>[3x]PMFIVNTNVPRASVPDGFLSELTQQLAQATGKPPQYIAVHVVPDQFMAFGGSSEPCALCSLHSIGKIGGAQNRSYSKLLCGLLAERLRISPDRVYINYYDMNAANVGWNNSTFA

Macrophage Migration Inhibitory Factor (MIF) is a ubiquitous multifunctional protein and a key player in the inflammatory response and innate immunity. MIF has two enzymatic activities: an evolutionarily well conserved keto-enol tautomerase activity and a thiol-protein oxido-reductase activity that is mediated by the C56ALC59 motif. X-ray structural studies have consistently shown that MIF exists as a homotrimer. Each MIF monomer consists of 114 amino acids and is composed of two anti-parallel α-helices packed against a four-stranded β-sheet.

To elucidate the role of intersubunit interactions involving Leu46 on the structure and stability of MIF, we compared the structural stability, and biophysical properties of wt, L46A, L46F and L46G mutants at the secondary, tertiary and quaternary structure levels. To understand the role of Leu46 mutations on the three-dimensional structure of MIF, we also determined the crystal structures of L46F, L46A and L46G huMIF at 1.70 Å, 1.70 Å and 1.60 Å, respectively. Similar to the wild type species, Leu46 mutants crystallized as homotrimeric proteins with dimensions of approximately 35 Å×50 Å×50 Å. In agreement with our previous structural studies, X-ray crystal structures of MIF variants demonstrate that the Leu46 mutants conserve the same three-dimensional structure pattern as the wt protein. Static light scattering, in agreement with the analytical ultracentrifugation data, demonstrated that wt, L46F, L46A and L46G exist as stable trimers. Finally, crystallographic data and enzymatic assays do not show any drastic conformational change of the catalytic site or activity of MIF upon Leu46 mutations. Using hydroxyphenylpyruvate as a substrate, we showed that all Leu46 mutants are enzymatically active. In our case, chemical shift measurements demonstrate an extremely high similarity between L46A and L46G huMIF, whereas the L46F mutant exhibits a slightly different chemical shift pattern. Taken together, our data suggest that the intersubunit interactions involving the residue Leu46 play a key role in the structural stability of MIF and provide new insights into the role of a novel intersubunit hydrophobic pocket in modulating MIF’s conformation, stability, and potentially its receptor binding and biological activity.>MTPPHNYLAVIKVVGIGGGGVNAVNRMIEQGLKGVEFIAINTDAQALLMSDADVKLDVGRDSTRGLGAGADPEVGRKAAEDAKDEIEELLRGADMVFVTAGEGGGTGTGGAPVVASIARKLGALTVGVVTRPFSFEGKRRSNQAENGIAALRESCDTLIVIPNDRLLQMGDAAVSLMDAFRSADEVLLNGVQGITDLITTPGLINVDFADVKGIMSGAGTALMGIGSARGEGRSLKAAEIAINSPLLEASMEGAQGVLMSIAGGSDLGLFEINEAASLVQDAAHPDANIIFGTVIDDSLGDEVRVTVIAAG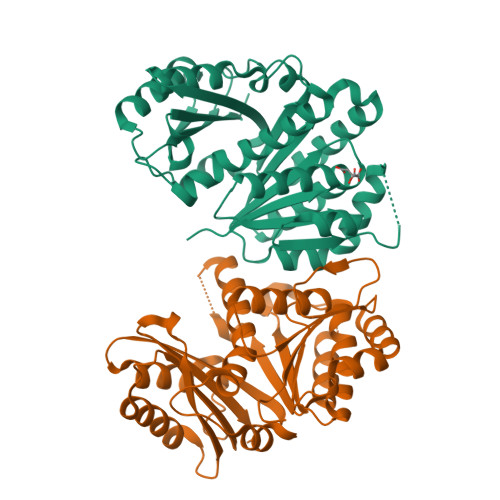FDVSGPGRKPVMGETGGAHRIESAKAGKLTSTLFEPVDAVSVPLHTNGATLSIGGDDDDVDVPPFMRR[2x]Scribble is a highly conserved regulator of cell polarity, a process that enables the generation of asymmetry at the cellular and tissue level in higher organisms. Scrib belongs to the LAP (leucine-rich repeats and PDZ domain) protein family, and features sixteen LLRs (Leucine-rich repeats), two LAP-specific domains (LAPSDa and LAPSDb) and the four PDZ domains (PDZ1, PDZ2, PDZ3 and PDZ4). The influenza A virus NS1 protein was shown to bind to human Scribble (SCRIB) via its C-terminal PDZ binding motif (PBM). Examination of the SCRIB PDZ:NS1 complexes showed that the NS1 peptides are bound in the canonical ligand-binding groove formed by the β2 strand and helix α2.

We determined crystal structures of SCRIB PDZ1 bound to NS1 ESEV PBM (A281-R219-T220-I221-E222-S223-E224-V225), SCRIB PDZ1 bound to NS1 ESKV PBM (A281-R219-T220-I221-E222-S223-K224-V225) and PDZ3 bound to NS1 ESKV PBM (A281-R219-T220-I221-E222-S223-K224-V225). The SCRIB PDZ1:ESEV complex revealed hydrogen bonds between Ser223ESEV-Ile742SCRIB PDZ1, Glu222ESEV-Ser762SCRIB PDZ1 and Ile223ESEV-Gly744SCRIB PDZ1. It appears that the conserved His in each domain found on the α2 helix, PDZ1 H793, PDZ3 H1071 and PDZ4 H1170A is an important position even when this was not obvious from the SCRIB PDZ1:ESEV structure, whereas in the SCRIB PDZ1:ESKV and SCRIB PDZ3:ESKV complexes a clear role for this His could be identified. In the case of the SCRIB PDZ1:ESEV complex, this is possibly due to the crystallographic packing (resulting in a different rotamer for the Ser 223 position in ESEV compared to ESKV), which prevents the Ser hydroxyl group from reaching SCRIB PDZ1 H793 for a hydrogen bond in the SCRIB PDZ1:ESEV complex. However, this interaction may be available in solution, since substitution of the His by an Ala significantly impacts the affinity of the interaction. The PDZ1 mutant H793A abolished binding with both the ESEV and ESKV PBM. The ESEV sequence showed an affinity towards all four SCRIB PDZ domains, with SCRIB PDZ4 showing the highest affinity interaction (KD = 11.8 ± 5.5 µM), followed by SCRIB PDZ3 (KD = 13.1 ± 1.6 µM), SCRIB PDZ2 (KD = 18.7 ± 2.4 µM) and lastly SCRIB PDZ1 (KD = 21.4 ± 1.7 µM). SCRIB PDZ1 displays a higher affinity to β-PIX (3.3 ± 0.3 µM), compared to both NS1 ESEV (21.4 ± 1.7 µM) and ESKV (30.0 ± 0.9 µM) PBMs. SCRIB PDZ1:ESEV and SCRIB PDZ1:ESKV superimposed with SCRIB PDZ1:β-PIX with RMSD values of 0.77 and 0.75 Å, respectively. The −1 position of β-PIX N645 forms a hydrogen bond with S741PDZ1, whereas the NS1 PBM does not interact with SCRIB PDZ1 from the −1 position; instead, the −2 position S223 appears to be the important position, forming a hydrogen bond with I742PDZ1.

>[2x]SAPSVKGVSFDQANNLLIEPARIEEEELTLTILRQTGGLGISIAGGKGSTPYKGDDEGIFISRVSEEGPAARAGVRVGDKLLEVNGVALQGAEHHEAVEALRGAGTAVQMRVWRERM;>ARTIESEV[2x]>[2x]GEIQWMRPSKEVGYPIINAPSKTKLEPSAFHYVFEGVKEPAVLTKNDPRLKTDFEEAIFSKYVGNKITEVDEYMKE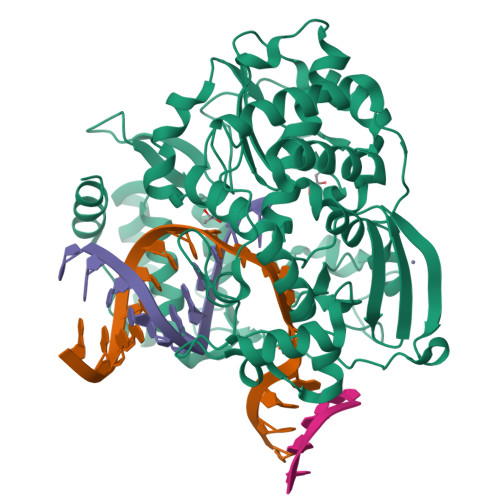AVDHYAGQLMSLDINTEQMCLEDAMYGTDGLEALDLSTSAGYPYVAMGKKKRDILNKQTRDTKEMQKLLDTYGINLPLVTYVKDELRSKTKVEQGKSRLIEASSLNDSVAMRMAFGNLYAAFHKNPGVITGSAVGCDPDLFWSKIPVLMEEKLFAFDYTGYDASLSPAWFEALKMVLEKIGFGDRVDYIDYLNHSHHLYKNKTYCVKGGMPSGCSGTSIFNSMINNLIIRTLLLKTYKGIDLDHLKMIAYGDDVIASYPHEVDASLLAQSGKDYGLTMTPADKSATFETVTWENVTFLKRFFRADEKYPFLIHPVMPMKEIHESIRWTKDPRNTQDHVRSLCLLAWHNGEEEYNKFLAKIRSVPIGRALDLPEYSTLYRRWLDSFGSSSHHHHHH> GPLGSVVRAKFNFQQTNEDELSFSKGDVIHVTRVEEGGWWEGTH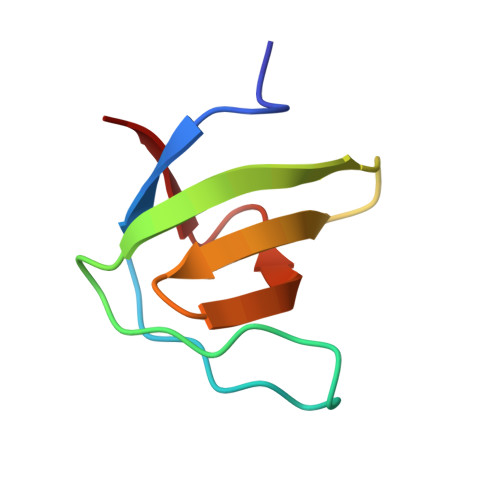NGRTGWFPSNYVREI> MHKFTGVNAKFQQPALRNLSPVVVEREREEFVGFFPQIVRDLTEDGIGHPEVGDAVARLKEVLQYNAPGGKCNRGLTVVAAYRELSGPGQKDAESLRCALAVGWCIELFQAASLVADDIMDQSLTRRGQLCWYKKEGVGLDAINDSFLLESSVYRVLKKYCRQRPYYVHLLELFLQTAYQTELGQMLDLITAPVSKVDLSHFSEERY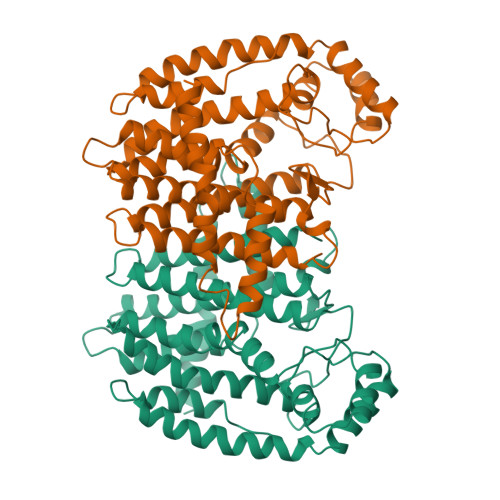KAIVKYKTAFYSFYLPVAAAMYMVGIDSKEEHENAKAILLEMGEYFQIQDDYLDCFGDPALTGAVGTDIQDNKCSWLVVQCLQRVTPEQRQLLEDNYGRKEPEKVAKVKELYEAVGMRAAFQQYEESSYRRLQELIEKHSNRLPKEIFLGLAQKIYKRQK> ETPPRFTRTPVDQTGVSGGVASFICQATGDPRPKIVWNKKGKKVSNQRFEVIEFDDGSGSVLRIQPLRTPRDEAIYECVASNNVGEISVSTRLTVLREDQIPRGFPTIDMGPQLKVVERTRTATMLCAASGNPDPEITW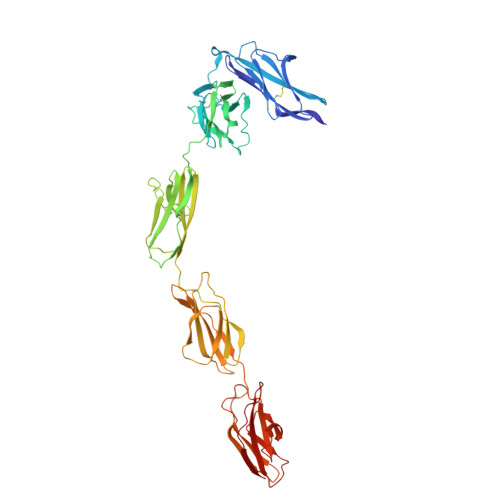FKDFLPVDTSNNNGRIKQLRSESIGGTPIRGALQIEQSEESDQGKYECVATNSAGTRYSAPANLYVRELREVRRVPPRFSIPPTNHEIMPGGSVNITCVAVGSPMPYVKWMLGAEDLTPEDDMPIGRNVLELNDVRQSANYTCVAMSTLGVIEAIAQITVKALPKPPGTPVVTESTATSITLTWDSGNPEPVSYYIIQHKPKNSEEPYKEIDGIATTRYSVAGLSPYSDYEFRVVAVNNIGRGPASEPVLTQTSEQAPSSAPRDVQARMLSSTTILVQWKEPEEPNGQIQGYRVYYTMDPTQHVNNWMKHNVADSQITTIGNLVPQKTYSVKVLAFTSIGDGPLSSDIQVIT>[2x]MKFDPQKYRELAEKDFEAAWKAGKEILAERSPNELYPRVGFSFGKEHPLFATIQRLREAYLSIGFSEVVNPLIVEDVHVKKQFGREALAVLDRCFYLATLPKPNVGISAEKIRQIEAITKREVDSKPLQEIFHRY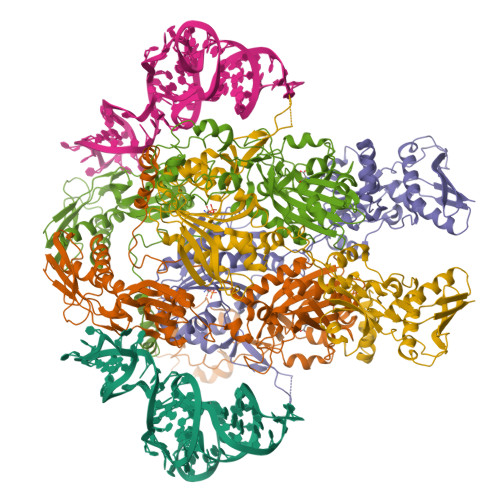KKGEIDGDDLSYLIAEVLDVDDITAVKILDEVFPEFKELKPISSTLTLRSHMTTGWFITLSHIADKLPLPIKLFSIDRCFRREQGEDATRLYTYFSASCVLVDEELSVDDGKAVAEALLRQFGFENFRFRKDEKRSKYYIPDTQTEVFAFHPKLVGSSTKYSDGWIEIATFGIYSPTALAEYDIPYPVMNLGLGVERLAMILYGYDDVRKMVYPQIHGEIKLSDLDIAREIKVKEVPQTAVGLKIAQSIVETAEKHASEPSPCSFLAFEGEMMGRNVRVYVVNENENTKLCGPAYANEVVVYKGDIYGIPKTKKWRSFFEEGVPTGIRYIDGFAYYAARKVEEAAMREQEEVKVKARIVENLSDINLYIHENVRRYILWKKGKIDVRGPLFVTVKAEIE4-(4-oxidanylidene-1'-propan-2-yl-spiro[3~{H}-chromene-2,4'-piperidine]-6-yl)-~{N}-(phenylmethyl)benzamide | C30 H32 N2 O3 | 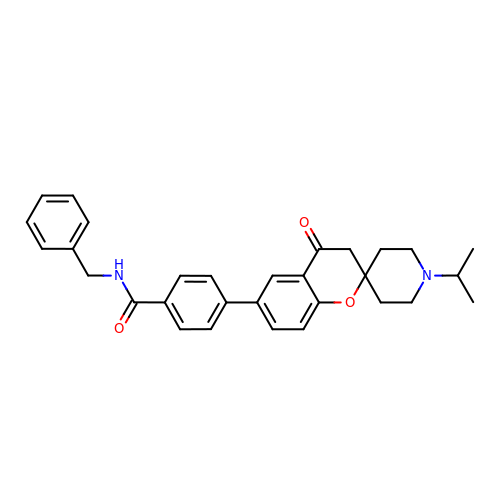ZNZGCTIEADJNIM-UHFFFAOYSA-N>[24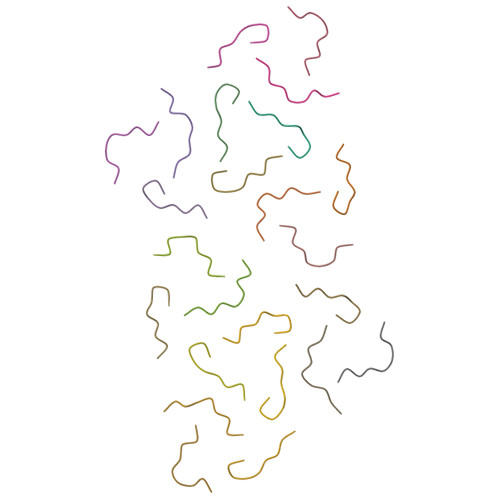x]GFGGNDNFG> TSFAPTVKICENLSQMSFAAREVILAAIDARVDKSVPVVLALSGGSTPKRLYEELHEKDLALLQQHAVQFILGDERLLSEDDEQSNFSMATKALLRDVPSSDVISIDRRAALATSKDEKGGLDGAWAVAQDYEVKL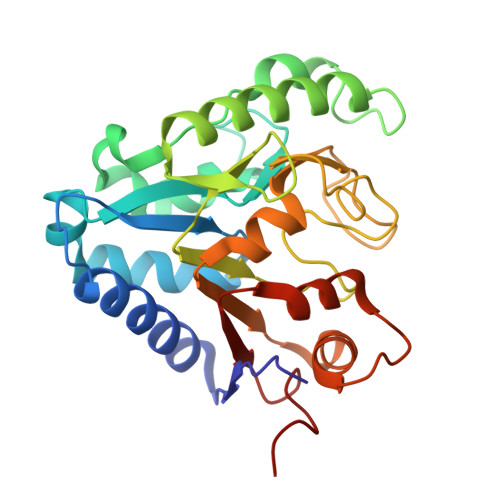LNCLPCKQINGTAKSVPVVDIVLLGFGSDGHTASIFPDSVAATDEEHVVSVSFPSPTMSPKVWRVTLSKTVIQYAKHVVVLAAGKDKNWVVRGVLSESPTDPLPVSRFLRDCRGSVTLLLDPGAGEGVCA>TPQNITDLCAEYHNTQIHTL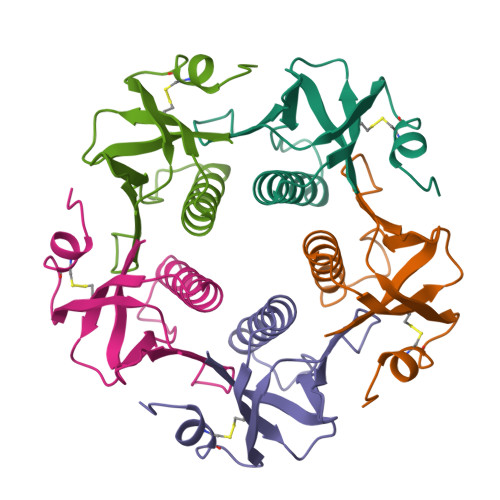NDKIFSYTESLAGKDEMAIITFKNGATFQVEVPGSQHIDSQKKAIERMKDTLRIAYLTEAKVEKLCVWNNKTPHAIAAISMAN[5x]> SDNAIAMEAAHSKSTEECLAYFGVSETTGLTPDQVKRHLEKYGHNELPAEEGKSLWELVIEQFEDLLVRILLLAACISFVLAWFEEGEETITAFVEPFVILLILIANAIVGVWQERNAENAIEALKEYEPEMGKVYRADRKSVQRIKARDIVPGDIVEVAVGDKVPADIRILSIKSTTLRVDQSILTGESVSVIKHTEPVPDPRAVNQDKKNMLFSGTNIAAGKALGIVATTGVSTEIGKIRDQMAATEQDKTPLQQKLDEFGEQLSKVISLICVAVWLINIGHFNDPVHGGSWIRGAIYYFKIAVALAVAAIPAGLPAVITTCLALGTRRMAKKNAIVRSLPSVETLGCTSVICSDKTGTLTTNQMSVCKMFIIDKVDGDFCSLN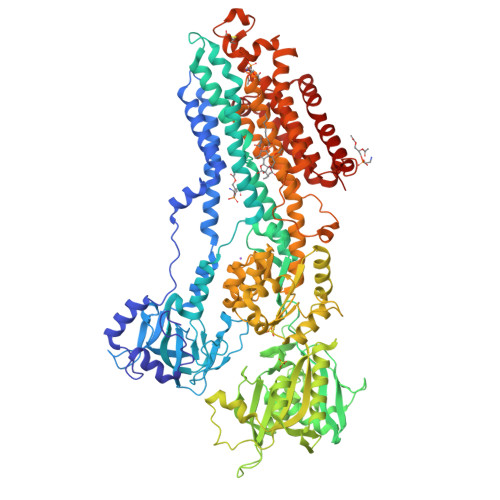EFSITGSTYAPEGEVLKNDKPIRSGQFDGLVELATICALCNDSSLDFNETKGVYEKVGEATETALTTLVEKMNVFNTEVRNLSKVERANACNSVIRQLMKKEFTLEFSRDRKSMSVYCSPAKSSRAAVGNKMFVKGAPEGVIDRCNYVRVGTTRVPMTGPVKEKILSVIKEWGTGRDTLRCLALATRDTPPKREEMVLDDSSRFMEYETDLTFVGVVGMLDPPRKEVMGSIQLCRDAGIRVIMITGDNKGTAIAICRRIGIFGENEEVADRAYTGREFDDLPLAEQREACRRACCFARVEPSHKSKIVEYLQSYDEITAMTGDGVNDAPALKKAEIGIAMGSGTAVAKTASEMVLADDNFSTIVAAVEEGRAIYNNMKQFIRYLISSNVGEVVCIFLTAALGLPEALIPVQLLWVNLVTDGLPATALGFNPPDLDIMDRPPRSPKEPLISGWLFFRYMAIGGYVGAATVGAAAWWFMYAEDGPGVTYHQLTHFMQCTEDHPHFEGLDCEIFEAPEPMTMALSVLVTIEMCNALNSLSENQSLMRMPPWVNIWLLGSICLSMSLHFLILYVDPLPMIFKLKALDLTQWLMVLKISLPVIGLDEILKFIARNYLEG>MTNIQKRFYKGRVALNVLANNIENAKDIFEAAEGYVVVGVLSKDYPTVEEAVTAMKAYGKEIDDAVSIGLGAGDNRQAAVVAEIAKHYSGSHINQVFPSVGATRANLGGKDSWINSLVSPTGKVGYVNISTGPISAAGEEKAIVPIKTAIALVRDMGGNSLKYFPMKGLAHEEEYRAVAKACAEEGF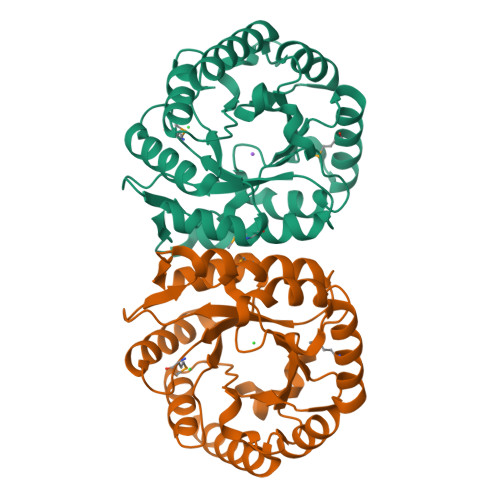ALEPTGGIDKENFETILRIALEANVEQVIPHVYSSIIDKETGNTKTEDVRELLAVVKKLVDQYA[2x]> MDLPEIVASGDPVLHEKAR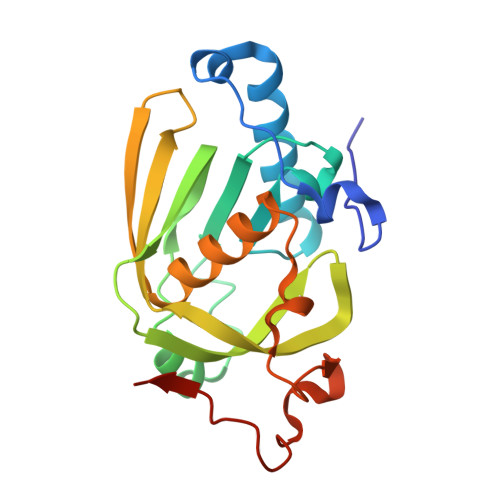EVDPGEIGSERIQKIIDDMIKVMRLAPGVGLAAPQIGVPLRIIVLEDTKEYISYAPKEEILAQERRHFDLMVMVNPVLKERSNKKALFFEGCLSVDGFRAAVERYLEVVVTGYDRQGKRIEVNASGWQARILQHECDHLDGNLYVDKMVPRTFRTVDNLDLPLAEGCPKLGSHHHHHH>MAVEPFPRRPITRPHASIEVDTSGIGGSAGSSEKVFCLIGQAEGGEPNTVYELRNYSQAKRLFRSGELLDAIELAWGSNPNYTAGRILAMRIEDAKPASAEIGGLKITSKIYGNVANNIQVGLEKNTLSDSLRLRVIFQDDRFNEVYDNIGNIFTIKYKGEEANATFSVEHDEETQKASRLVLKVGDQEVKSYDLTGGAYDYTNAIITDINQLPDFEAKLSPFGDKNLESSKLDKIENANIKDKAVYVKAVFGDLEKQTAYNGIVSFEQLNAEGEVPSNVEVEAGEESATVTATSPIKTIEPFELTKLKGGTNGEPPATWADKLDKFAHEGGYYIVPLSSKQSVHAEVASFVKERSDAGEPMRAIVGGGFNESKEQLFGRQASLSNPRVSLVANSGTFVMDDGRKNHVPAYMVAVALGGLASGLEIGESITFKPLRVSSLDQIYESIDLDELNENGIISIEFVRNRTNTFFRIVDDVTTFNDKSDPVKAEMAVGEANDFLVSELKVQLEDQFIGTRTINTSASIIKDFIQSYLGRKKRDNEIQDFPAEDVQVIVEGNEARISMTVYPIRSFKKISVSLVYK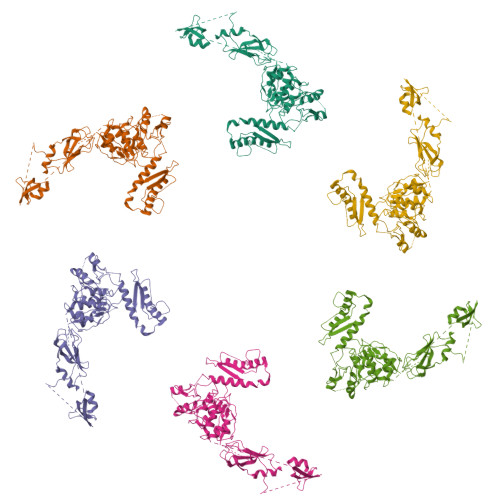QQTLQA[6x]>MDNKTYEISSAEWEVMNIIWMKKYASANNIIEEIQMQKDWSPKTIRTLITRLYKKGFIDRKKDNKIFQYYSLVEESDIKYKTSKNFINKVYKGGFNSLVLNFVEKEDLSQDEIEELRNILNKK[2x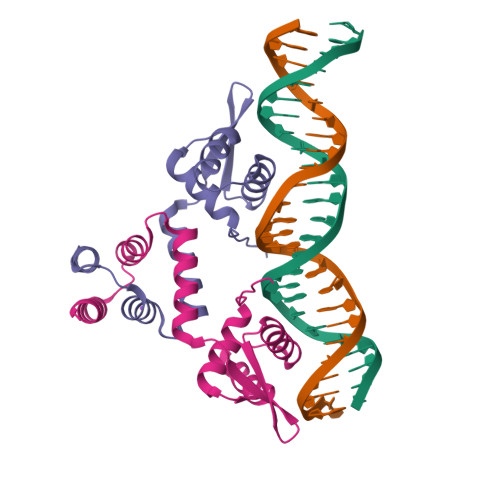]>[2x]GAMEEKYLPELMAEKDSLDPSFTHALRLVNQEIEKFQKGEGKDEEKYIDVVINKNMKLGQKVLIPVKQFPKFNFVGKLLGPRGNSLKRLQEETLTKMSILGKGSMRDKAKEEELRKSGEAKYFHLNDDLHVLIEVFAPPAEAYARMGHALEEIKKFLIPDYN

T-STAR is a tissue-specific STAR protein mainly expressed in the testis and brain3426, and regulates the alternative splicing of CD44, Tra2β, Tau, VGEF and Neurexin pre-mRNAs262728. STAR proteins are defined by the presence of a highly conserved RNA-binding domain, the STAR domain, also responsible for homodimerization, and composed of a central KH (K homology) domain flanked by two highly conserved regions, QUA1 and QUA2. Here, we have determined the X-ray structures of the T-STAR KH domain in its free state, and in complex with AAAUAA; KH-QUA2 in complex with AAUAAU; QUA1-KH in complex with UAAU; and the full STAR domain in complex with AUUAAA. Taken together, our data reveal a unique mode of RNA recognition and dimerization by the STAR proteins Sam68 and T-STAR that is crucial for their function in alternative splicing.

The structures of the T-STAR QUA1-KH and STAR domains in complex with RNA show that the QUA1 and the KH domains form compact dimers, with each KH domain binding one RNA molecule, while the QUA2 domain does not adopt a fixed orientation. The QUA1 domain adopts a helix-turn-helix motif involved in homodimerization, and its fold is very similar to the structure of isolated Sam68 QUA1 reported previously (backbone root mean square deviation (RMSD) of 0.61 Å). No electron density could be observed for the N-terminal half of the linker connecting the QUA1 to the KH domain (residues 35–42), suggesting that this region is disordered, while the C-terminal half of the linker (residues 43–53) is well defined in the structures. Surprisingly, the KH domain and the C-terminal half of the QUA1-KH linker of T-STAR provide an additional dimerization interface. This novel KH/linker interface covers 1,065 Å2 per monomer, almost twice as large as the QUA1 dimerization interface, and involves mainly the C-terminal α-helix 3 of the KH domain and the C-terminal half of the QUA1-KH linker. The KH interface is stabilized by a network of hydrophobic interactions involving residues A138, Y141, M144, G145 and L148, and an intermolecular hydrogen bond between Y141 in α-helix 3 and Q58 in β-strand 1 of the KH. The C-terminal half of the QUA1-KH linker (residues 43–53) also contributes to the dimer interface with the side chain of Y45 and the backbone of I46, forming a network of hydrogen bonds with the side chain of D125 and the backbone atoms of K59 and L61. Accordingly, the structure of T-STAR STAR in complex with AUUAAA overlay very well with the structure of T-STAR QUA1-KH in complex with UAAU with a backbone RMSD of 0.9 Å for the QUA1-KH atoms. The crystal structures of T-STAR QUA1-KH and STAR domains show that the QUA1 dimer contacts only one KH domain. From our NMR and SAXS data in solution, we conclude that the contacts between the QUA1 dimer and one KH domain observed in our X-ray structures are most probably due to crystal packing.> MPIYPIEGLSPYQNRWTIKARVTSKSDIRHWSNQRGEGKLFSVNLLDDSGEIKATGFNDAVDRFYPLLQENHVYLISKARVNIAKKQFSNLQNEYEITFENSTEIEECTDATDVPEVKYEFVRINELESVEANQQCDVIGILDSYGELSEIVSKASQRPVQKRELTLVDQGNRSVKLTLWGKTAETFPTNAGVDEKPVLAFKGVKVGDFGGRSLSMFSSSTMLINPDITESHVLRGWYDNDGAHAQFQPYTNGGVGGGAMGGGGAGANMAERRTIVQVKDENLGMSEKPDYFNVRATVVYIKQEN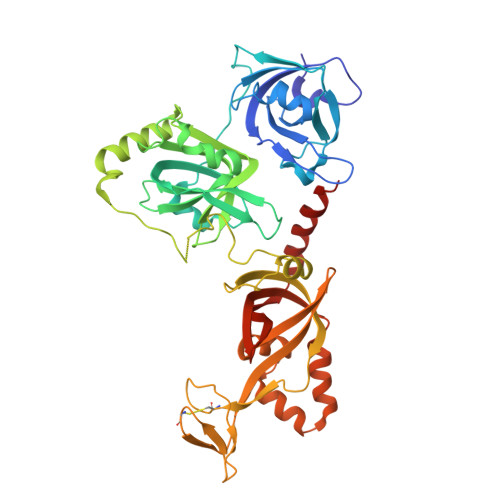LYYTACASEGCNKKVNLDHENNWRCEKCDRSYATPEYRYILSTNVADATGQMWLSGFNEDATQLIGMSAGELHKLREESESEFSAALHRAANRMYMFNCRAKMDTFNDTARVRYTISRAAPVDFAKAGMELVDAIRAYM>MNNTIETILAHRSIRKFTAVPITDEQRQTIIQAGLAASSSSMLQVVSIVRVTDSEKRNELAQFAGNQAYVESAAEFLVFCIDYQRHATINPDVQADFTELTLIGAVDSGIMAQNCLLAAESMGLGGVYIGGLRNSAAQVDELLGLPENSAVLFGMCLGHPDQNPEVKPRLPAHVVVHENQYQE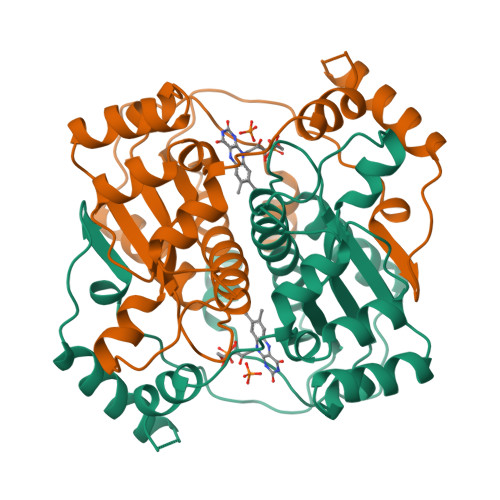LNLDDIQSYDQTMQAYYASRTSNQKLSTWSQEVTGKLAGESRPHILPYLNSKGLAKR[2x]> GVDNAEKGKVSNDDASVDFVAEPVKLPENQTRVAFFYDRAVPIGMLRPGQNMETTFNYQENDYRLNCLLLTPLP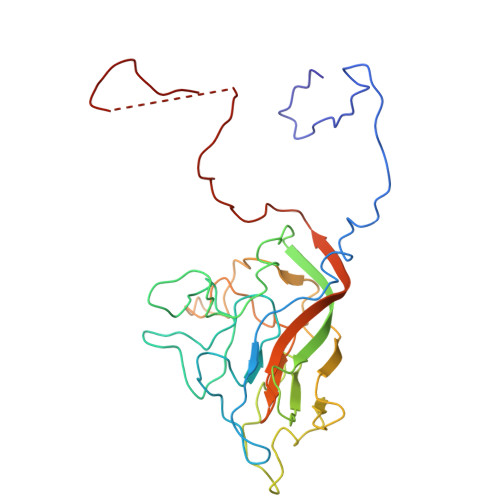SFCPDSSSGPQKTKAPVQWRWVRSGGVNGANFPLMTKQDYAFLCFSPFTFYKCDLEVTVSALGTDTVASVLRWAPTGAPADVTDQLIGYTPSLGETRNPHMWLVGAGNSQVSFVVPYNSPLSVLPAAWFNGWSDFGNTKDFGVAPNADFGRLWIQGNTSASVRIRYKKMKVFCPRPTLFFPWPTPTTTKINADNPVPILELE> ATIPSESPFAAAEVADGAIVVDIAKMKYETPELHVKVGDTVTWINREAMPHNVHFVAGVLGEAALKGPMMKKEQAYSLTFTEAGTYDYHCTPHPF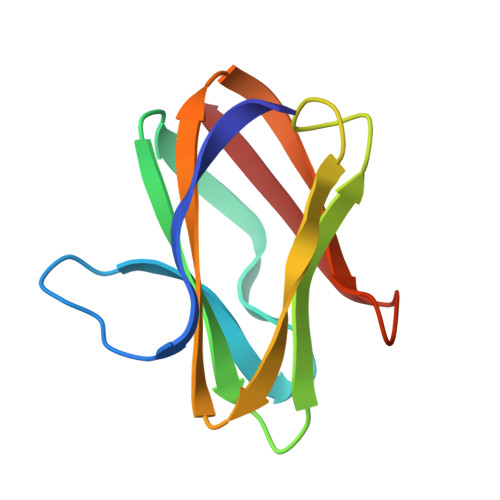MRGKVVVE> GAMSETSVNRGPEKIRPECFELLRVLGKGGYGKVFQVRKVTGANTGKIFAMKVLKKAMIVRNAKDTAHTKAERNILEEVKHPFIVDLIYAFQTGGKLYLILEYLSGGELFMQLEREGIFMEDTACFYLAEISMALGHLHQKGIIYRDLKPENIMLNHQGHVKLTDFGLCKESIHDGTVT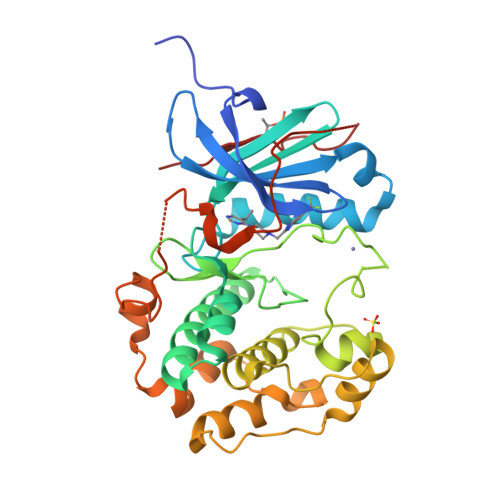HTFCGTIEYMAPEILMRSGHNRAVDWWSLGALMYDMLTGAPPFTGENRKKTIDKILKCKLNLPPYLTQEARDLLKKLLKRNAASRLGAGPGDAGEVQAHPFFRHINWEELLARKVEPPFKPLLQSEEDVSQFDSKFTRQTPVDSPDDSTLSESANQVFLGFTYVAPS>[2x]AMGSRKSKAELQSEERKRIDELIESGKEEGMKIDLIDGKGRGVIATKQFSRGDFVVEYHGDLIEITDAKKREALYAQDPST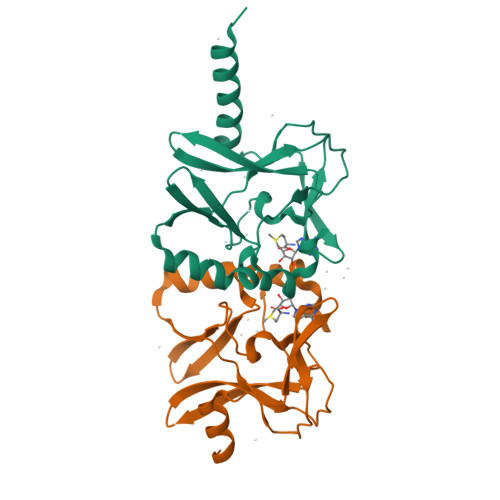GCYMYYFQYLSKTYCVDATRETNRLGRLINHSKSGNCQTKLHDIDGVPHLILIASRDIAAGEELLYDYGDRSKASIEAHPWLKH> QFAKPEDAVKYRQSAVTLMASHFGRMTPVVKGQAPYDAAQIKANVEVLKTLSALPWAAFGPGTEGGDARPEIWSDAASFKQKQQAFQDNIVKLSAAADAGDL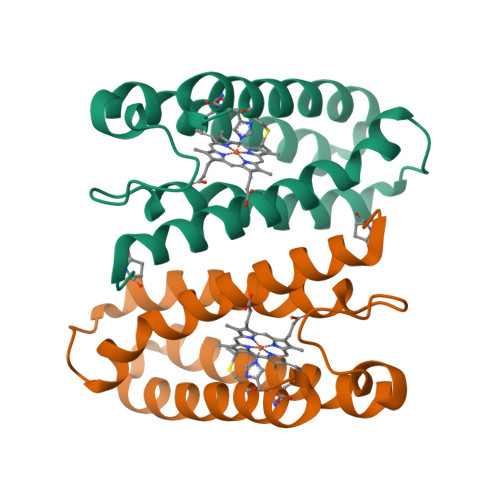DKLRAAFGDVGASCKACHDAYRKK> MEDTPLVISKQKTEVVCGVPTQVVCTAFSSHILVVVTQFGKMGTLVSLEPSSVASDVSKPVLTTKVLLGQDEPLIHVFAKNLVAFVSQEAGNRAVLLAVAVKDKSMEGLKALREVIRVCQVW

There is considerable evidence that the assembly of the eukaryotic 26S proteasome does not proceed spontaneously, but is mediated by several assembly chaperones. The formation of the 20S CP is assisted by five proteasome-specific chaperones: PAC1–PAC4 and POMP in humans; Pba1–Pba4 and Ump1 in yeast. Recently reported knock-out experiments indicated that α4, α5, α6, and α7 form a core assembly intermediate as part of the initial process of α-ring assembly, which is supported by PAC3-PAC4. In summary, we produced structural insights into the functional mechanisms of the PAC3-PAC4 heterodimer as a molecular matchmaker underpinning the α4-α5-α6 subcomplex during α-ring formation.

In addition, we newly determined a 0.96-Å high-resolution trigonal structure of the PAC3 homodimer. The overall structure of the trigonal form was very similar to that of the tetragonal structure we have previously published, except for a loop comprised of residues 51–61, suggesting that it is mobile. Loop flexibility was also observed in the corresponding segment of the yeast ortholog Pba3 in its heterodimer with Pba4. Our nuclear magnetic resonance (NMR) relaxation data from the human PAC3 homodimer confirmed that the loop is indeed mobile and disordered in solution. A complex model, model A, based on the 2.00-Å PAC3 structure showed that the mobile loop was turned toward the solvent. Another model based on the 0.96-Å structure, model B, showed that the corresponding loop contacts α6. Apart from interactions involving this mobile loop, intermolecular contacts between the PAC3-PAC4 heterodimer and the proteasomal subunits are almost identical in the two models. Specifically, Ser55, Lys80, and Asn81 of PAC3 form hydrogen bonds or electrostatic interactions with Ser110, Asp94, and Arg96 of α6, respectively. There are also predicted hydrophobic interactions of Val61, Phe85, and Val77 in PAC3 with Phe87, Phe97, and Leu93 in α6. Therefore, despite the low sequence similarity, the overall interaction modes of the matchmaking chaperones with the proteasomal subunits appear to be conserved between humans and yeast. It is plausible that the conformational flexibility of the mobile 51–61 loop of PAC3, which carries the α6-contacting residues, contributes to the interaction adjustability.> MGVLITGCGSRGDTEPLVALAARLRELGADARMCLPPDYVERCAEVGVPMVPVGRAVRAGAREPGELPPGAAEVVTEVVAEWFDKVPAAIEGCDAVVTTGLLPAAVAVRSMAEKLGIPYRYTVLSPDHLPSEQSQAERDMYNQGADRLFGDAVNSHRASIGLPPVEHLYDYGYTDQPWLAADPVLSPLRPTDLGTVQTGAWILPDQRPLSAELEGFLRAGSPPVYVGFGSGPAPAEAARVAIEAVRAQGRRVVLSSGWAGLGRIDEGDDCLVVGEVNHQVLFGRVAAVVHHGGAGTTTAVTRAGAP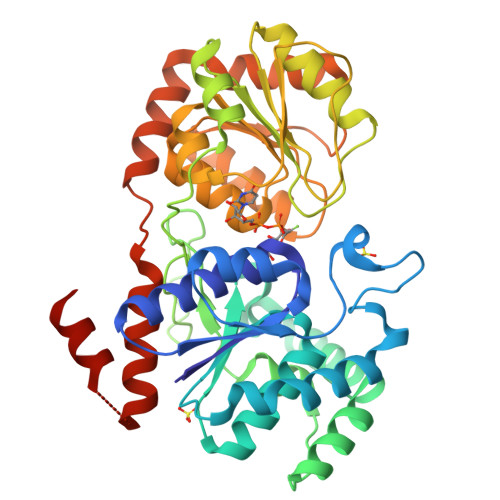QVVVPQKADQPYYAGRVADLGVGVAHDGPTPTVESLSAALATALTPGIRARAAAVAGTIRTDGTTVAAKLLLEAISRQRSSVPAAKLAAALEHHHHHH> GAMAERSLLTGEEGWRTYKATGPALSLPALVALLKGQGLEVGKVA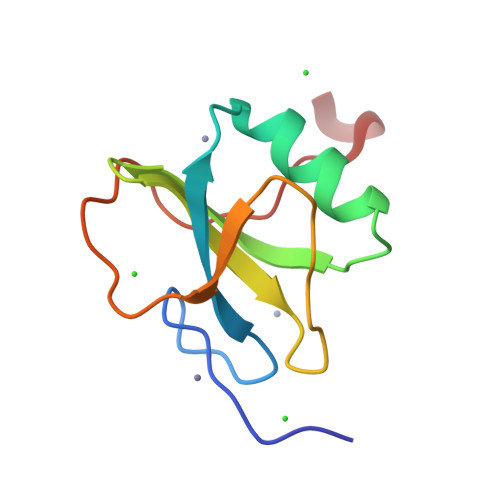EAEGGFYVDLRPEARPEVAGLRLEPARRVEGLLEIPSRTRRPARA> MANYPHTPTQAAKRRKETLMLQKLRNRKGFTLIELLIVVAIIGILAAIAIPQFSAYRVKAYNSAASSDLRNLKTALESAFADDQTYPPES;> MKKIITIVAMLLAMQGIAIAAGKIPTTTMGGKDFTFKPSTNVSVSYFTTNGATSTAGTVNTDYAVNTK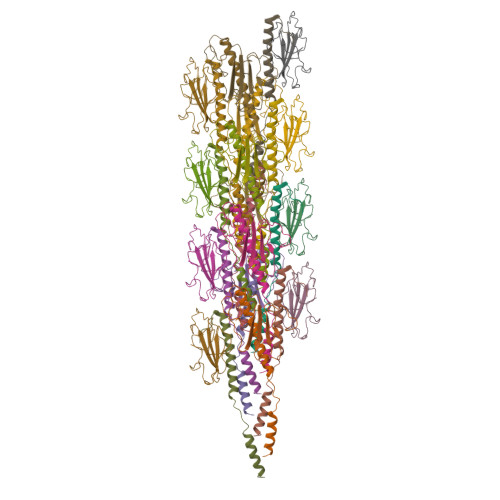NSSGNRVFTSTNNTSNIWYIENDAWKGKAVSDSDVTALGTGDVGKSDFSGTEWKSQ>MKAPVRVAVTGAAGQIGYSLLFRIAAGEMLGKDQPVILQLLEIPQAMKALEGVVMELEDCAFPLLAGLEATDDPDVAFKDADYALLVGAAPRKAGMERRDLLQVNGKIFTEQGRALAEVAKKDVKVLVVGNPANTNALIAYKNAPGLNPRNFTAMTRLDHNRAKAQLAKKTGTGVDRIRRMTVWGNHSSTMFPDLFHAEVDGRPALELVDMEWYEKVFIPTVAQRGAAIIQARGASSA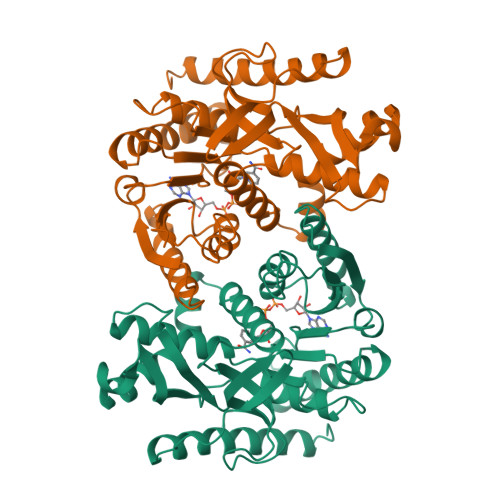ASAANAAIEHIRDWALGTPEGDWVSMAVPSQGEYGIPEGIVYSFPVTAKDGAYRVVEGLEINEFARKRMEITAQELLDEMEQVKALGLI[2x]(5-hydroxy-4-{[(1-hydroxy-7-methoxy-2-oxo-1,2-dihydroquinolin-3-yl)amino]methyl}-6-methylpyridin-3-yl)methyl 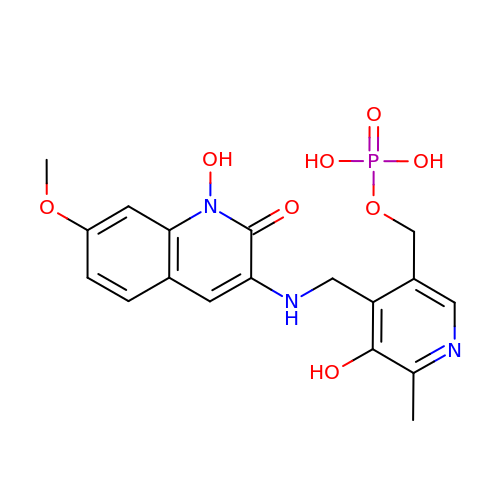dihydrogen phosphate | C18 H20 N3 O8 P | QSKPSFPICSGYQC-UHFFFAOYSA-N The highly oxidising protein DsbA catalyses disulfide bond formation between two cysteine residues of unfolded substrates in the periplasm of Gram-negative bacteria. The structure of DsbA is comprised of a thioredoxin domain with an inserted helical domain. Like many other thiol-disulfide oxidoreductase enzymes, the active site of DsbA is comprised of the characteristic CXXC motif (Cys30–Pro31–His32–Cys33 in Escherichia coli DsbA) and a highly conserved cis-proline in an adjacent loop which has been shown to play a key role in the binding of substrates. Adjacent to the active site is a hydrophobic groove which serves as a site for both DsbB and unfolded substrates to form a complex.

As the crystal structure of the p-anisidine analogue 16 showed that the installation of the p-methoxy group induced a shift of the benzofuran core away from His32 (relative to anilino 15), the m-methoxy substituted phenyl ether 26 was synthesised to observe whether the shift could be avoided. The co-structure showed a horizontal rotation relative to the unsubstituted phenoxy 25 (comparable to 16) but notably a less pronounced shift into the left-hand side of the binding groove, meaning the π-stacking interaction between the benzofuran core and His32 could be better retained. The m-methoxy group of 26 may potentially form a polar interaction with side chain of Gln35, although electron density for this compound was insufficient to unambiguously define the interaction. The addition of a m-methoxy 26 substituent on the 6-phenoxy group led to a 2-fold decrease in binding affinity, while extending the phenoxy group to a benzyloxy group led to a 2.5-fold decrease. This suggests that 26 may not engage any polar interactions with DsbA despite its close proximity to the polar residues His32 and Gln35. Adding functional groups (16 and 26) or extending the ring linker increased the heavy atom count but did not contribute to binding affinity; therefore, leading to less efficient binders.

>AQYEDGKQYTTLEKPVAGAPQVLEFFSFFCPHCYQFEEVLHISDNVKKKLPEGVKMTKYHVNFMGGDLGKDLTQAWAVAMALGVEDKVTVPLFEGVQKTQTIRSASDIRDVFINAGIKGEEYDAAWNSFVVKSLVAQQEKAAADVQLRGVPAMFVNGKYQLNPQGMDTSNMDVFVQQYADTVKYLSEKK[2x]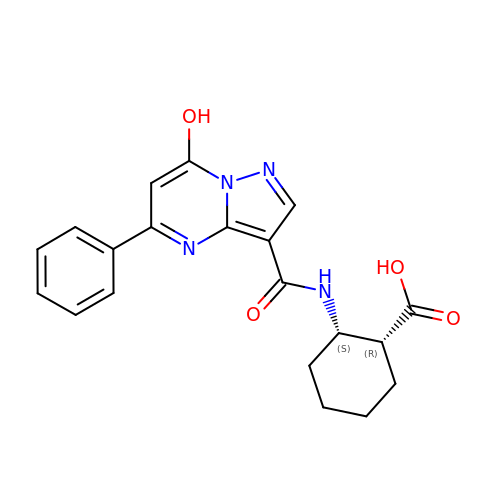(1R,2S)-2-[(7-hydroxy-5-phenylpyrazolo[1,5-a]pyrimidine-3-carbonyl)amino]cyclohexane-1-carboxylic acid | C20 H20 N4 O4 | PHGTYMRDHDEHLI-HIFRSBDPSA-N> GPLGSGKIMPNTVFVGGIDVRMDETEIRSF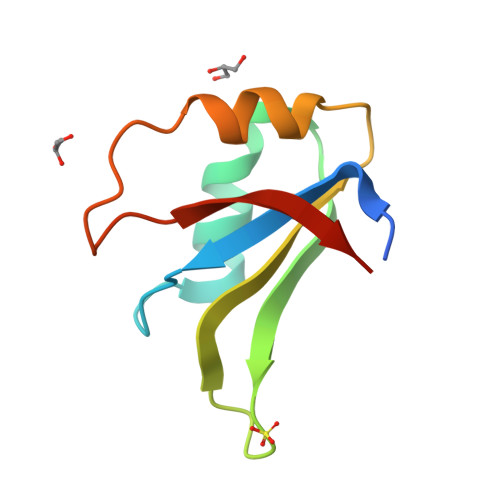FARYGSVKEVKIITDRTGVSKGYGFVSFYNDVDVQKIVESQINFHGKKLKLGPAIRKQN>VVGTFKAKDLIVTPAEILKEKPDPNNLVFGTVFTDHMLTVEWSSEFGWEKPHIKPLQNLSLHPGSSALHYAVELFEGLKAFRGVDNKIRLFQPNLNMDRMYRSAVRATLPVFDKEELLECIQQLVKLDQEWVPYSTSASLYIRPTFIGTEPSLGVKKPTKALLFVLLSPVGPYFSSGTFNPVSLWANPKYVRAWKGGTGDCKMGGNYGSSLFAQCEAVDNGCQQVLWLYGEDHQITEVGTMNLFLYWINEDGEEELATPPLDGIILPGVTRRCILDLAHQWGEFKVSERYLTMDDLTTALEGNRV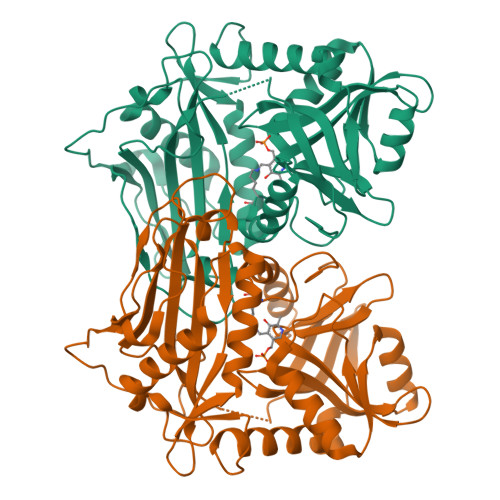REMFGSGTACVVCPVSDILYKGETIHIPTMENGPKLASRILSKLTDIQYGREERDWTIVL[2x]(2R)-2-((R)-CARBOXY{[CARBOXY(4-HYDROXYPHENYL)ACETYL]AMINO}METHOXYMETHYL)-5-METHYLENE-5,6-DIHYDRO-2H-1,3-OXAZINE-4-CARBOXYLIC 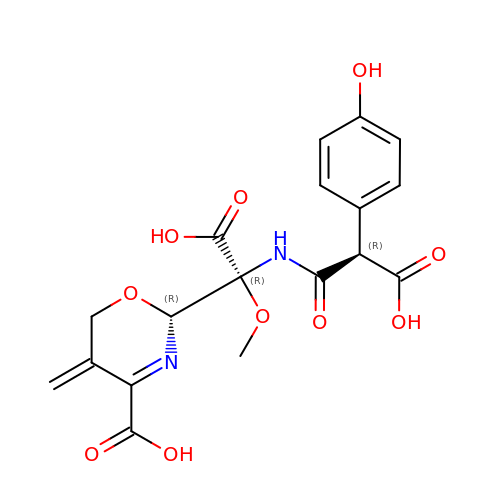ACID | C18 H18 N2 O10 | ZTOQXKUYWZBJLG-XNAIMREJSA-N> MVRIVIDSGVDSGRPIGVVPFQWAGPGAAPEDIGGIVAADLRNSGKFNPLDRARLPQQPGSAQEVQPAAWSALGIDAVVVGQVTPNPDGSYNVAYQLVDTGGAPGTVLAQNSYKVNKQWLRYAGHTASDEVFEKLTGIKGAFRTRIAYVVQTNGGQFPYELRVSDYDGYNQFVVHRSPQCLMSPAWSPDGSKLAYVTFESGR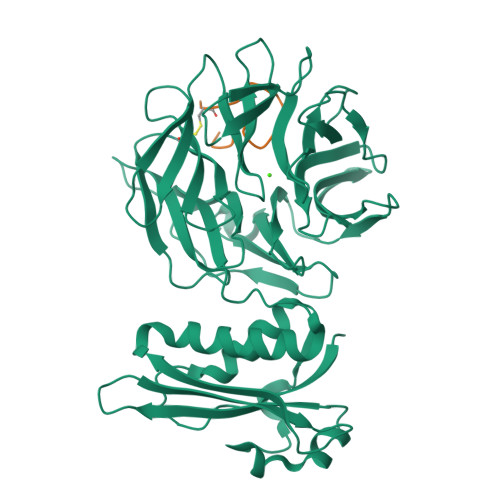SALVIQTLANGAVRQVASFPRHNGAPAFSPDGSKLAFALSKTGSLNLYVMDLASGQIRQVTDGRSNNTEPTWFPDSQNLAFTSDQAGRPQVYKVNINGGAPQRITWEGSQNQDADVSSDGKFMVMVSSNGGQQHIAKQDLATGGVQVLSSTFLDETPSLAPNGTMVIYSSSQGMGSVLNLVSTDGRFKARLPATDGQVKFPAWSPYLLEHHHHHH;> GCSDGSGWSSENNPWG>[4x]MAHHHHHHMKKAPTVSVIVAA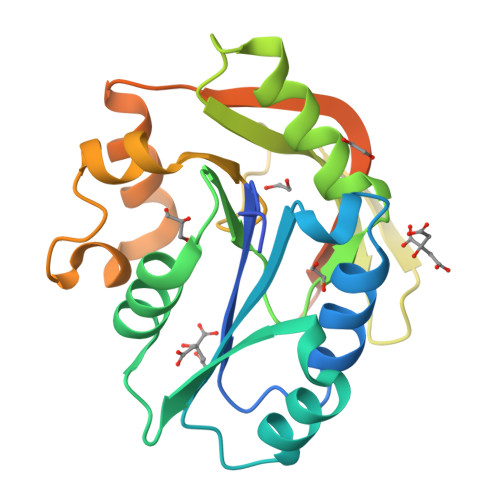FNQEKYIGRCIRSLLNQNFPKEDYEIIIINDGSTDKTKYALEIFGKEIKVIENESNKGLSASLNLGIRSALGQFIVRVDADDYVNSDYVSILHKFLSYNPNFDAVACDYYLVDDHEDFLSRKNCMIDPIGCGIMFRIEQLIDIGLYDDGFLSHEDKDLRIRFEKKYSIHRVELPLYRYRRHDSNMTNDSELMDERMKSLREKHKDQP>MGSDKIHHHHHHMKYGIVGYSGRMGQEIQKVFSEKGHELVLKVDVNGVEELDSPDVVIDFSSPEALPKTVDLCKKYRAGLVLGTTALKEEHLQMLRELSKEVPVVQAYNFSIGINVLKRFLSELVKVLEDWDVEIVETHHRFK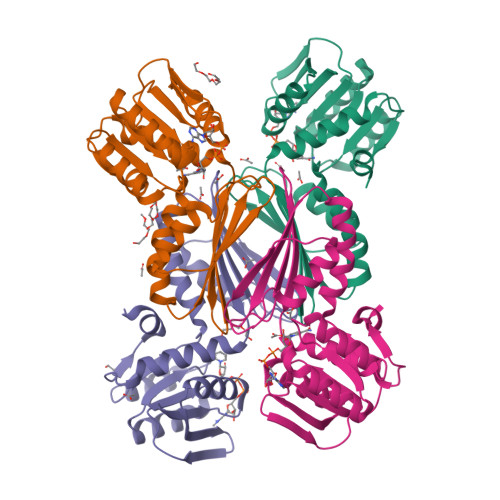KDAPSGTAILLESALGKSVPIHSLRVGGVPGDHVVVFGNIGETIEIKHRAISRTVFAIGALKAAEFLVGKDPGMYSFEEVIFGGE[4x]> MSKKLLFQFDTDATPSVFDVVVGYDGGADHITGYGNVTPDNVGAYVDGTIYTRGGKEKQSTAIFVGGGDMAAGERVFEAVKKRFFGPFRVSCMLDSNGSNTTAAAGVALVVKAAGGSVKGKKAVVLAGTGPVGMRSAALLAGEGAEVVLCGRKLDKAQAAADSVNKRFKVNVTAAETADDASRAEAVKGAHFVFTAGAIGLELLPQAAWQNESSIEIVADYNAQPPLGIGGIDATDKGKEYGGKRAFGALGIGG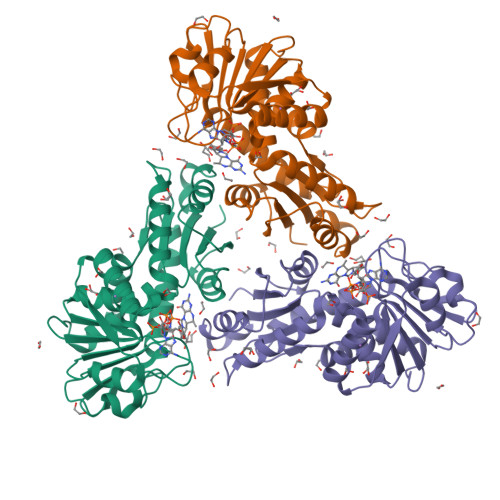LKLKLHRACIAKLFESSEGVFDAEEIYKLAKEMAVDKLAAALEHHHHHH> LLLQSPAVKFITNPEFFTVLHANYSAYRVFTSSTCLKHMILKVRRDARNFER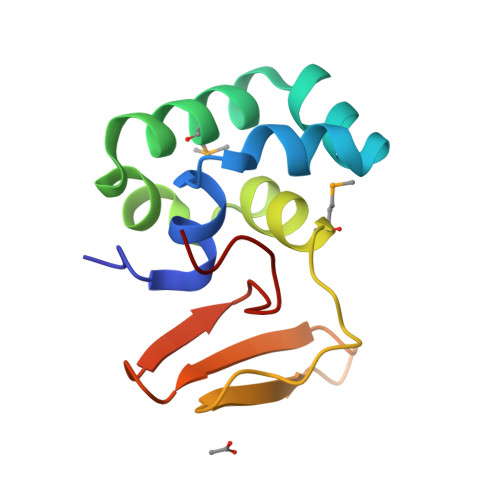YQHNRDLVNFINMFADTRLELPRGWEIKTDQQGKSFFVDHNSRATTFIDPRIPLQNG> MRKLNKKEEQRKASTENILGCALDLFVKNGYRATTIDMIAARAGLTKGAIYFYFKTKDAIMLMLLEEAEKYIVDPIDEYMANAGPLADAKLVKFINMQALLGVTKPQHVLLLILVSIDFSGTGDDIEKRAKAIYRRMYGHVEQLIAQGQTEGVFRSDSGSDELASIVMAAHDGVLIEWYRRPNELTGKTLTKALRSVLLNGL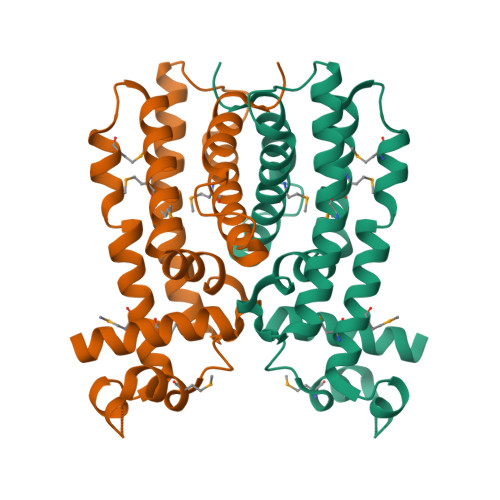IVDRGSCKNPTF> LPTDTTTFKRIFLKRMPSIRESLKERGVDMARLGPEW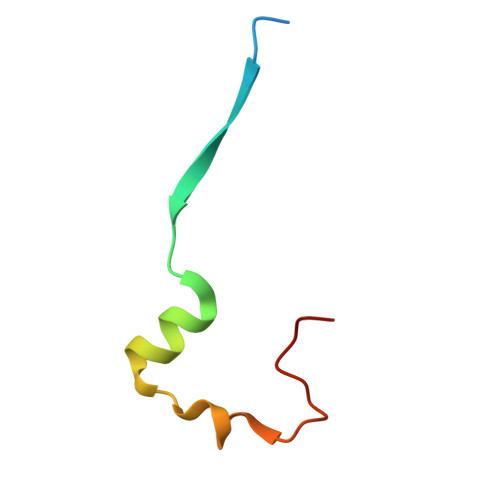SQPMKR> MGQLTQTNKTELGVFDDMNQAIEAAKEAQLVVKKMSMDQREKIISAIRKKTIEHAETLARMAVEETGMGNVGHKILKHQLVAEKTPGTEDITTTAWSGDRGLTLVEMGPFGVIGAITPCTNPSETIICNTIGMLAGGNTVVFNPHPAAIKTSNFAVQLINEASLSAGGPVNIACSVRKPTLDSSKIMMSHQDIPLIAATGGPGVVTAVLQSGKRGIGAGAGNPPVLVDETADIR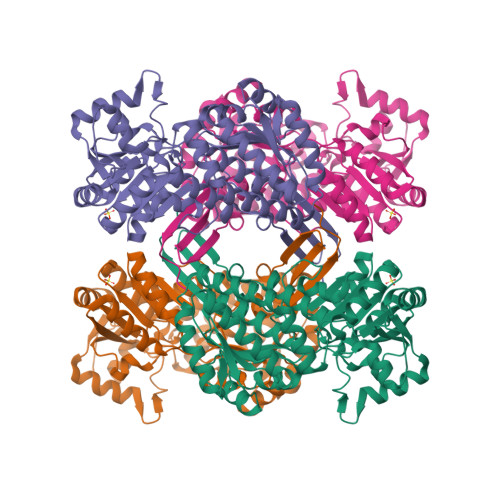KAAEDIINGCTFDNNLPCIAEKEVVAIDAIANELMNYMVKEQGCYAITKEQQEKLTNLVITPKGLNRNCVGKDARTLLGMIGIDVPSNIRCIIFEGEKEHPLISEELMMPILGIVRAKSFDDAVEKAVWLEHGNRASAHIHSKNVDRITTYAKAIDTAILVKNAPSYAAIGFGGEGFCTFTIASRTGEGLTSASTFTKRRRCVMSDSLCIR>[2x]MVRDKYYLITHGSQDPYWTSLFQGAKKAAEELKVDLQILAPPGANDVPKQVQFIESAL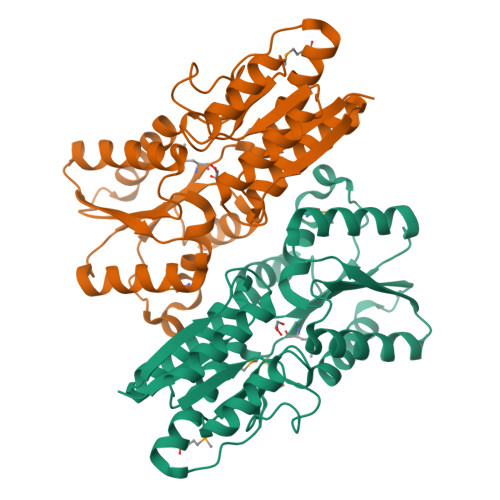ATYPSGIATTIPSDTAFSKSLQRANKLNIPVIAVDTRPKDKTKNPYLVFLGSDNLLAGKKLGEKALELTPSAKRALVLNPQPGHIGLEKRAYGIKTILQDKGIFFEELDVGTDPNQVQSRVKSYFKIHPETNIIFCLTSQALDPLGQMLLHPDRYDFNYQPQVYSFDKTPNTVSLIHKKLVNYVMDQQPFLMGYLSITQLVLMNRYQLNPVNINTAMAENLYFQSHHHHHHWSHPQFEK>[3x]ATAAEIAALPRQKVELVDPPFVHAHSQVAEGGPKVVEFTMVIEEKKIVIDDAGTEVHAMAFNGTVPGPLMVVHQDDYLELTLINPETNTLMHNIDFHAATGALGGGGLTEINPGEKTILRFKATKPGVFVYHCAPPGMVPWHVVSGMNGAIMVLPREGLHDGKGKALTYDKIYYVGEQDFYVPRDENGKYKKYEAPGDAYEDTVKVMR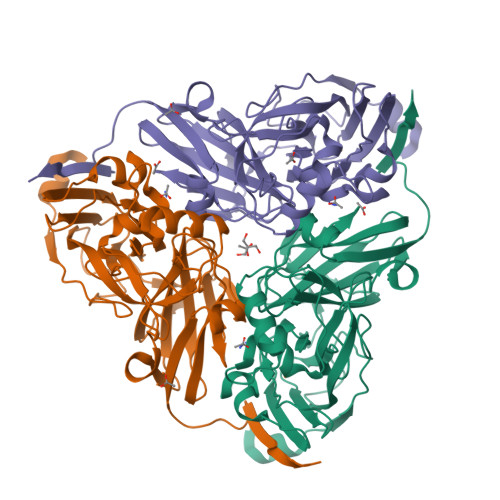TLTPTHVVFNGAVGALTGDKAMTAAVGEKVLIVHSQANRDTRPHLIGGHGDYVWATGKFNTPPDVDQETWFIPGGAAGAAFYTFQQPGIYAYVNHNLIEAFELGAAAHFKVTGEWNDDLMTSVLAPSGT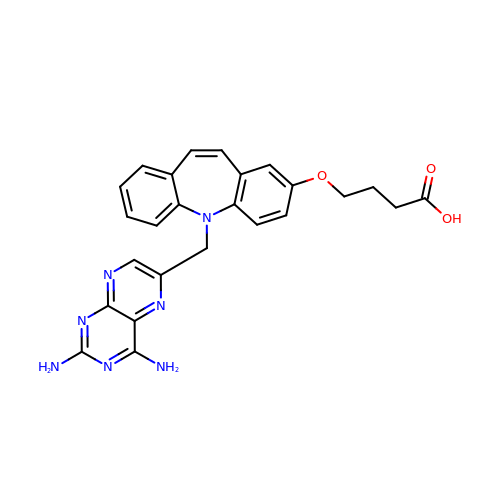4-({5-[(2,4-diaminopteridin-6-yl)methyl]-5H-dibenzo[b,f]azepin-2-yl}oxy)butanoic acid | C25 H23 N7 O3 | ORMJWSHZQMNLEH-UHFFFAOYSA-N> MKATEQHYSIKEAMLFSQRIAQLSKALWKSIEKDWQRWIKPFDLNINEHHILWIAYHFKGASISEIAKFGVMHVSTAFNFSKKLEEKGLLSFSKKQDDKRNTYIELTEKGEEVLMKLMETYDPTKNAVFNGALPLRELY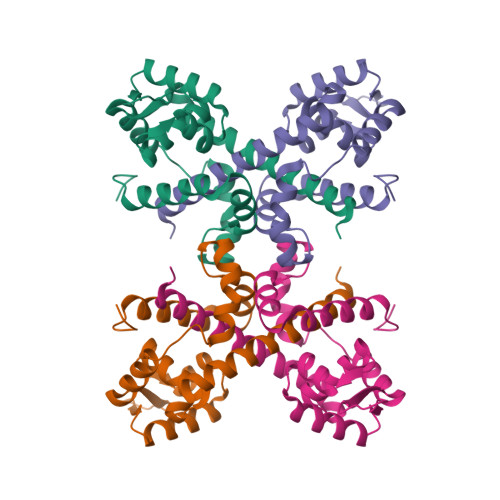GKFPEILEMMCIVRNIYGDDFMEIFERAFENIKEDFIEQDGKLVKRKPKTEEHEKELASQANHHHHHH glutaryl-coenzyme 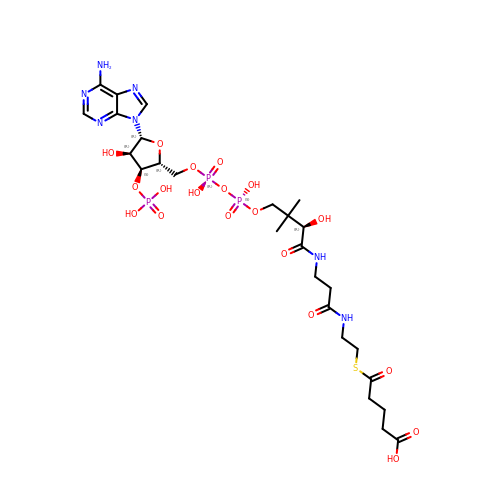A | C26 H42 N7 O19 P3 S | SYKWLIJQEHRDNH-CKRMAKSASA-N> MDPSKDSKAQVSAAEAGITGTWYNQLCSTFIVTAGADGALT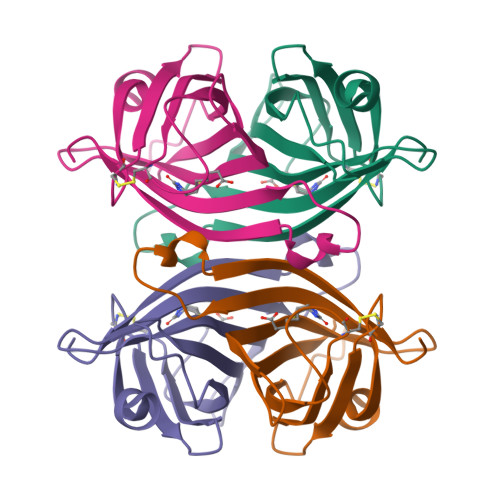GTYESCVGNAESRYVLTGRYDSAPATDGSGTALGWTVAWKNNYRNAHSATTWSGQYVGGAEARINTQWLLTSGTTEANAWKSTLVGHDTFTKVKPSAASIDAAKKAGVNNGNPLDAVQQ> SPQPLEQIKLSESQLSGRVGMIEMDLASGRTLTAWRADERFPMMSTFKVVLCGAVLARVDAGDEQLERKIHYRQQDLVDYSPVSEKHLADGMTVGELCAAAITMSDNSAANLLLATVGGPAGLTAFLRQIGDNVTRLDRWETELNEALPGDARDTTTPASMAATLRKLLTSQRLSARSQRQLLQWM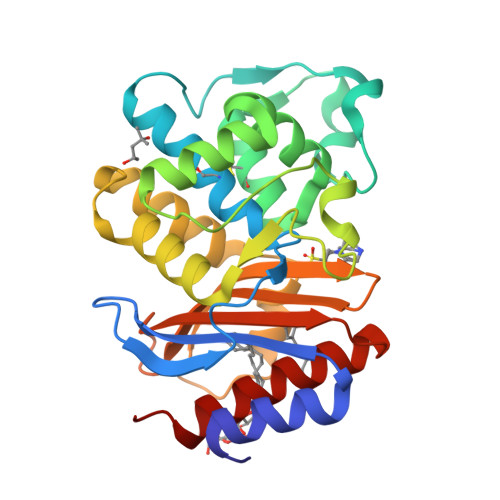VDDRVAGPLIRSVLPAGWFIADKTGASERGARGIVALLGPNNKAERIVVIYLRDTPASMAERNQQIAGIGAALIEHWQR The complex P. falciparum life cycle is supported by a diverse repertoire of surface proteins including the family of 6-Cys s48/45 antigens. Pf12, Pf38, Pf41 and Pf92 are localized on the surface of the blood-stage merozoite, which is the form of the parasite that invades erythrocytes, proliferates, and causes the symptoms of malaria. On the merozoite surface, Pf12 and Pf41 are displayed as a heterodimer with Pf12 tethered to the outer membrane via a glycophosphatidylinositol (GPI) anchor and soluble Pf41 appropriately localized through its interaction with Pf12. Collectively, these data establish the architectural organization of Pf41 and define an essential role for the Pf41 ID in promoting assembly of the Pf12-Pf41 heterodimeric complex.

To compensate for this innate property of Pf41, surface lysines were chemically methylated during purification, and crystals of methylated Pf41 were observed after eight months. Ultimately, the structure of Pf41 was determined by zinc single-wavelength anomalous dispersion to a resolution of 2.45 Å. One Pf41 molecule was present in the asymmetric unit, and PISA analysis indicated that Pf41 crystallized as a monomer consistent with a previous analysis showing no homo-multimerization capabilities. The refined model of Pf41 begins at Lys21 and extends through Glu369, with a four residue disordered region (Lys59 to Ser62) and an extended, un-modelled region between Ser137 and Ile224 (left). Two of the dimethylated lysines were located at a crystal packing interface (right), underscoring the importance of lysine methylation in obtaining diffraction quality crystals of Pf41. Structural analysis confirms that both Pf41 6-Cys domains (D1 and D2) adopt a β-sandwich fold with expected disulfide connectivity of C1-C2, C3-C6 and C4-C5; the first two disulfides pin together the two sheets of the β-sandwich and the latter disulfide anchors an ancillary loop to the domain core. Intriguingly, despite a rotation of D1 relative to D2, the relative spatial positioning of the two 6-Cys domains of Pf41 is analogous to that of Pf12, with overall dimensions for these two domains of approximately 65 by 40 Å, despite the prediction that the 6-Cys domains of Pf41 are separated by a large spacer. Strikingly, structural analysis revealed that the additional residues in Pf41 map to three distinct regions: a large inserted domain-like region (ID) of 108 residues (Thr117 to Ile225) between the β8 and β9 strands of the D1 core that is largely proteolyzed in the final structure, the D1 β9 strand, and the short inter-domain linker. Analysis of the crystal packing revealed insufficient room in the crystal lattice to accommodate the un-modelled residues leading us to conclude that the region was proteolyzed during the extended time frame in which it took the crystals to form.

> GSMGKSHKCDFTKEKYLLSGEKEVSCEIDANPADDITFICPNKIDSLCFHTVNIAKNINQNKATMSIQDLLYGSVVYGNTLFISPYVRTNTPFYCFCNLDTVTIQKFLKINRFLKDDDELSEADVMKHLKGGNVAEAQADEYLNKALNRFKKMKDLSKFFNDQADNTAKLNLPKSLNIPNDILNYDVYNSANNRNDIVVKDEVTNKQIISKRGIMSVFVRSNNNVIKGCDFGNNNKNYFSHPISVAGKVNNKVCKIQGKPGELVGFKCAFEENGKVEPPNCFDQVLHKNKVTDLKTLIPGYASYTNKHSSKYPYYLKIPHFVNEQYTIQCKCKSNNAQNEYTFELDIQPGESEVVLNSFKTSAAA> QTSVSPSKVILPRGGSVLVTCSTSCDQPKLLGIETPLPKKELLLPGNNRKVYELSNVQEDSQPMCYSNCPDGQSTAKTFLTVYWTPERVELAPLPSWQPVGKQLTLRCQVEGGAPRAQLTVVLLRGEKELKREPAVGEPA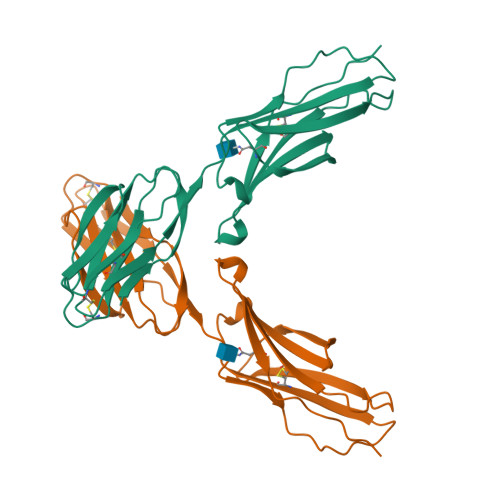EVTTTVLVRRDHHGAQFSCRTELDLRPQGLELFENTSAPYQLQTF> TAQK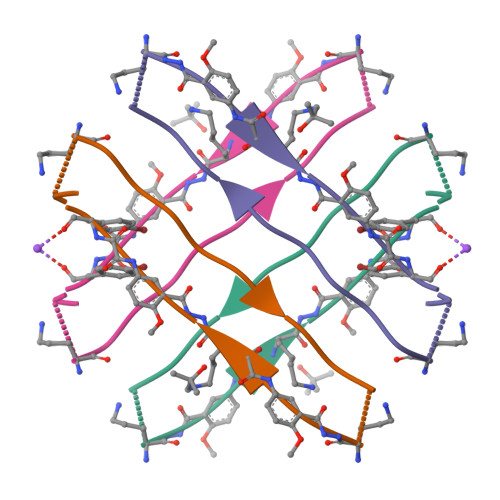LVFFAEDAXKXY>[2x]NTKYNKEFLLYLAGFVD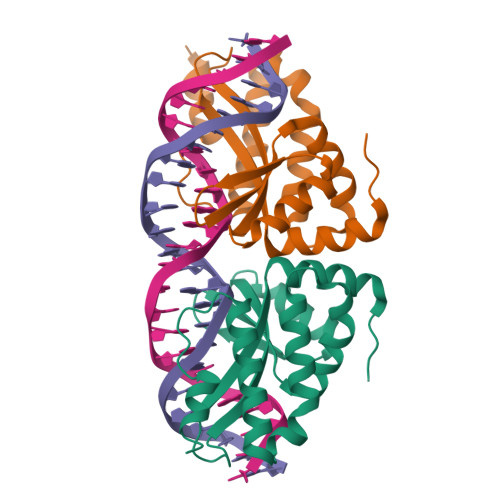GDGSIIAQIKPNQSYKFKHQLSLTFQVTQKTQRRWFLDKLVDEIGVGYVRDRGSVSNYILSEIKPLHNFLTQLQPFLKLKQKQANLVLKIIEQLPSAKESPDKFLEVCTWVDQIAALNDSKTRKTTSETVRAVLDS>[2x]MQQKLTSPDNNLVMTFQVDSKGAPTYELTYKNKVVIKPSTLGLELKKEDNTRTDFDWVDRRDLTKLDSKTNLYDGFEVKD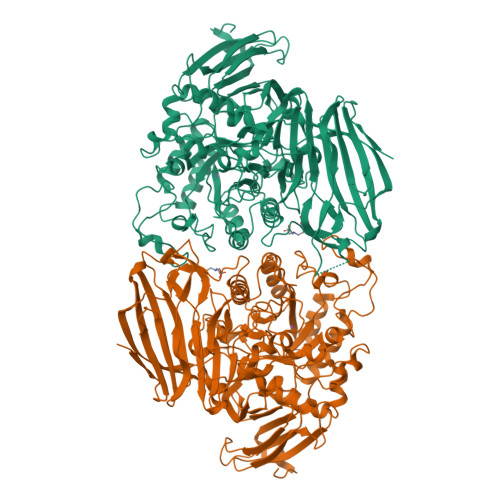TQTATFDETWQPVWGEEKEIRNHYNELAVTLYQPMNDRSIVIRFRLFNDGLGFRYEFPQQKSLNYFVIKEEHSQFGMNGDHIAFWIPGDYDTQEYDYTISRLSEIRGLMKEAITPNSSQTPFSQTGVQTALMMKTDDGLYINLHEAALVDYSCMHLNLDDKNMVFESWLTPDAKGDKGYMQTPCNTPWRTIIVSDDARNILASRITLNLNEPCKIADAASWVKPVKYIGVWWDMITGKGSWAYTDELTSVKLGETDYSKTKPNGKHSANTANVKRYIDFAAAHGFDAVLVEGWNEGWEDWFGNSKDYVFDFVTPYPDFDVKEIHRYAARKGIKMMMHHETSASVRNYERHMDKAYQFMADNGYNSVKSGYVGNIIPRGEHHYGQWMNNHYLYAVKKAADYKIMVNAHEATRPTGICRTYPNLIGNESARGTEYESFGGNKVYHTTILPFTRLVGGPMDYTPGIFETHCNKMNPANNSQVRSTIARQLALYVTMYSPLQMAADIPENYERFMDAFQFIKDVALDWDETNYLEAEPGEYITIARKAKDTDDWYVGCTAGENGHTSKLVFDFLTPGKQYIATVYADAKDADWKENPQAYTIKKGILTNKSKLNLHAANGGGYAISIKEVKDKSEAKGLKRLLEHHHHHH> MDFTSDTTNSHDTSNSHLSLEDAVGTHHAGEADVNIDGDEKQQLSLLDDDQVRALKLQEEKDALLTRRNTLLQEIQTYQNILMKENNSKTKNGDILQNDITQDFLNLISISSSNPNSAISDRKRVERINGLTNLQKELVTKYDTLPLLNMNLRLSYLRDHTYPHLQVSVQSRDRVHNDGIEVLVVNYKFCRNTMNPFEIQFKMFYKFEDSTLLKWEILRISTNVRLKAKQLLATRNFQKCLLSLYEFDKIKSKKTGIFQNLINLLKRKTRCYLMNNSDSLIVERVIREGRLTTIKLQINFIITMPGERGKPRNCFLPMSKISIALWKGGERFNQIDLDEICYGLIKEYGVK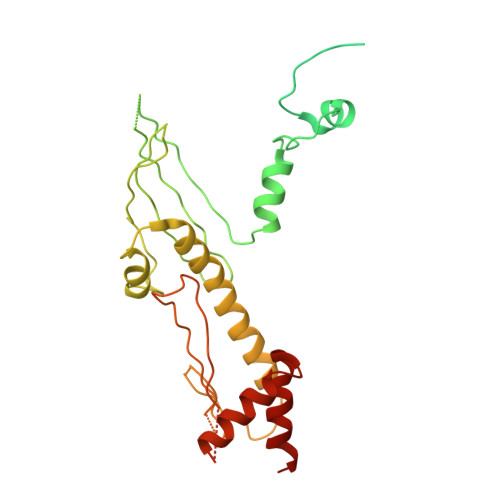TGLKEICNVCLFPDMYAR(2-AMINO-2,3-DIHYDRO-1H-INDEN-2-YL)PHOSPHONIC 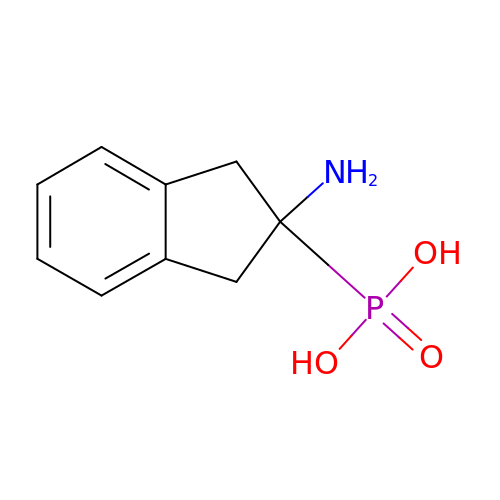ACID | C9 H12 N O3 P | YJFRDRWPYDVEIH-UHFFFAOYSA-N>[4x]MQRERLEKVMSSHTPKLDSCGAEPIHIPGAIQEHGALL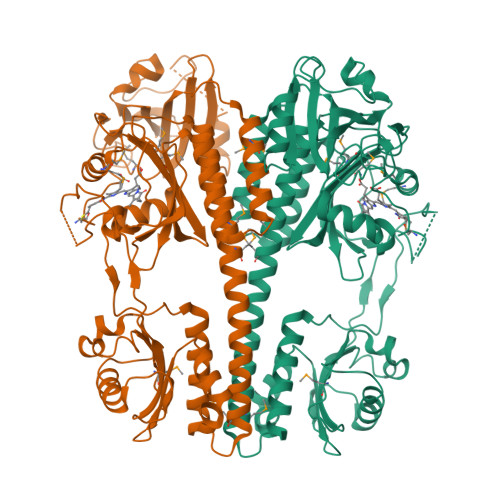VLSAREFSVVQASDNLANYIGVDLPIGAVATEANLPFISVLSAWYSGEESNFRYAWAEKKLDVSAHRSGTLVILEVEKAGVGESAEKLMGELTSLAKYLNSAPSLEDALFRTAQLVSSISGHDRTLIYDFGLDWSGHVVAEAGSGALPSYLGLRFPAGDIPPQARQLYTINRLRMIPDVDYKPVPIRPEVNAETGAVLDMSFSQLRSVSPVHLEYMRNMGTAASMSVSIVVNGALWGLIACHHATPHSVSLAVREACDFAAQLLSMRIAMEQSSQDASRRVELGHIQARLLKGMAAAEKWVDGLLGGEGEREDLLKQVGADGAALVLGDDYELVGNTPSREQVEELILWLGEREIADVFATDNLAGNYPTAAAYASVASGIIAMRVSELHGSWLIWFRPEVIKTVRWGGDPHKTVQESGRIHPRKSFEIWKEQLRNTSFPWSEPELAAARELRGAIIGIVLRKTEEHHHHHH>[2x]MSSTTLHNAMQYTAFDVLSSILNLMKADP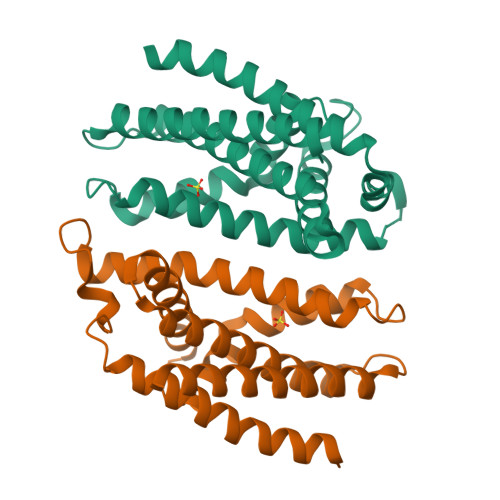LYDLLQLNQAYSSQDQEYEKNEFYGDSYLEERASSLVLKFLRKYEQIPFEMYSGLRIHTVKNQTLGEIFDLLHLGDTKTFEKKKKGDLVESLIGGCVLLSQRENATLFLLFAHALIDYIFYHSSYIYFNANPPKLVKEEIITDIQNWFKDKLFYYRSSLEKYQTDP> MMKRNILAVIVPALLVAGTANAAEIYNKDGNKVDLYGKAVGLHYFSKGNGENSYGGNGDMTYARLGFKGETQINSDLTGYGQWEYNFQGN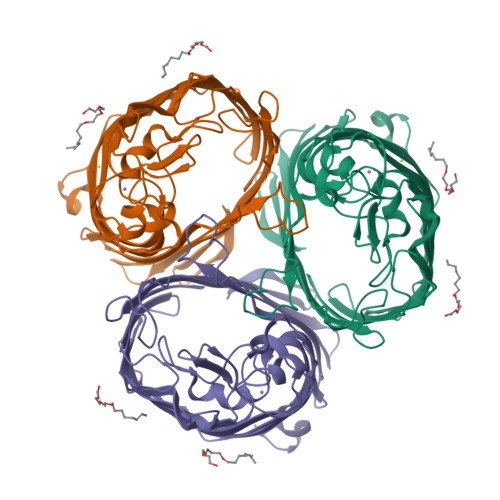NSEGADAQTGNKTRLAFAGLKYADVGSFDYGRNYGVVYDALGYTDMLPEFGGDTAYSDDFFVGRVGGVATYRNSNFFGLVDGLNFAVQYLGKNERDTARRSNGDGVGGSISYEYEGFGIVGAYGAADRTNLQEAQPLGNGKKAEQWATGLKYDANNIYLAANYGETRNATPITNKFTNTSGFANKTQDVLLVAQYQFDFGLRPSIAYTKSKAKDVEGIGDVDLVNYFEVGATYYFNKNMSTYVDYIINQIDSDNKLGVGSDDTVAVGIVYQF> MLSRRYAAKSFVEWYYRQINENKPVASGYVNNNATYTKAGHPPADITINGRVVATPEEWDTMLKEQRAQHNTSSSSTLPIGRKPVRYDVDCFDVHVINADYRFAAPQRMIEQHAPTDGVRMMMALTVSGSVYFGASPRSTDDYVIKQHFNDVFILVPNWDVLEKPGARS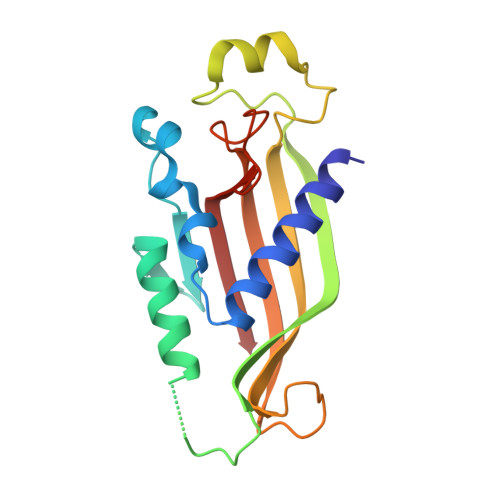GRKYLIASHKYRAY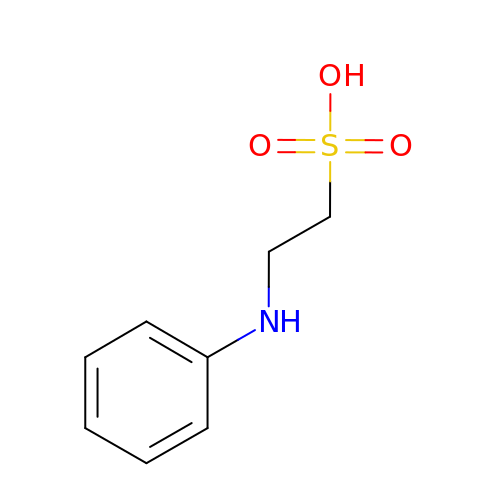2-PHENYLAMINO-ETHANESULFONIC ACID | C8 H11 N O3 S | IAVHKMVGTPXJIC-UHFFFAOYSA-N>MKHHHHHHPMGATTQYTTLPSVLLIGPSGAGKTALLTLFERGPLLNPDGTSVGAADLKNPYRKPIVTSPVAQTHTSQVPTSVELAVGANEDGTPTSYKVDLDAAGATARKFLLIDTPGHPKLRGTTLQHLLNPSPSLTIIPTNAPNKKTSTDSHSDPYKSKLKAVIFLLDAAALADSDGDYLSQTASYLYDVLLSLQKRFHSRKNSRAPSSIPVLIAANKQDLFTAVPASLVKSRLEHELGRIRKTRQKGLLEASVTSEDEIRADDEEGWLGAVGSKEFKFEEMMEFDMEVEVMGGNVIG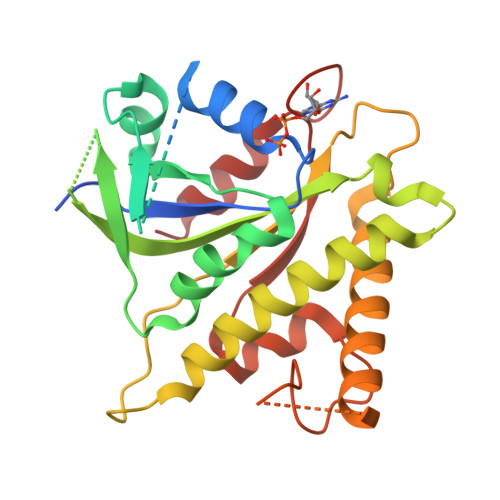DGPGAERWWRWIGERI[2x]>AEGQTNADDTLVVEASTPSLYAPQQSADPKFSRPVADTTRTMTVISEQVIKDQGATNLTDALKNVPGVGAFFAGENGNSTTGDAIYMRGADTSNSIYIDGIRDIGSVSRDTFNTEQVEVIKGPSGTDYGRSAPTGSINMISKQPRNDSGIDASASIGSAWFRRGTLDVNQVIGDTTAVRLNVMGEKTHDAGRDKVKNERYGVAPSVAFGLGTANRLYLNYLHVTQHNTPDGGIPTIGLPGYSAPSAGTAALNHSGKVDTHNFYGTDSDYDDSTTDTATMRFEHDINDNTTIRNTTRWSRVKQDYLMTAIMGGASNITQPTSDVNSWTWSRTANTKDVSNKILTNQTNLTSTFYTGSIGHDVSTGVEFTRETQTNYGVNPVTLPAVNIYHPDSSIHPGGLTRNGANANGQTDTFAIYAFDTLQITRDFELNGGIRLDNYHTEYDSATACGGSGRGAITCPTGVAKGSPVTTVDTAKSGNLMNWKAGALYHLTENGNVYINYAVSQQPPGGNNFALAQSGS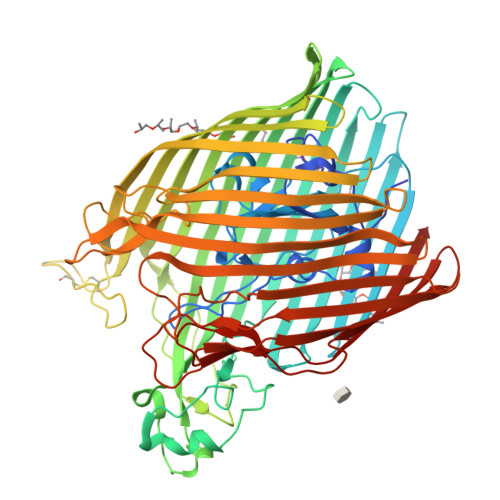GNSANRTDFKPQKANTSEIGTKWQVLDKRLLLTAALFRTDIENEVEQNDDGTYSQYGKKRVEGYEISVAGNITPAWQVIGGYTQQKATIKNGKDVAQDGSSSLPYTPEHAFTLWSQYQATDDISVGAGARYIGSMHKGSDGAVGTPAFTEGYWVADAKLGYRVNRNLDFQLNVYNLFDTDYVASINKSGYRYHPGEPRTFLLTANMHF[2x]~{N}-[3,5-bis(chloranyl)phenyl]-4-methyl-3-[(1-methyl-6-pyridin-3-yl-pyrazolo[3,4-d]pyrimidin-4-yl)amino]benzamide 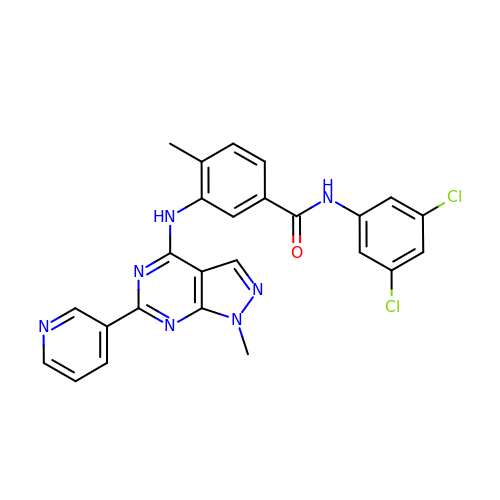| C25 H19 Cl2 N7 O | MTFBPWRBMAVOLM-UHFFFAOYSA-N Activins, members of transforming growth factor β (TGF-β) superfamily, were first isolated from porcine ovarian follicular fluid and identified as activating factors for the release of follicle stimulating hormone. Activins function both in autocrine and paracrine manner. They conduce signalling by binding to extracellular domains of type I and type II receptors and allowing the kinase domains of type II receptors to phosphorylate those of type I receptors and initiate the intracellular signalling. Activins, like all other members in the TGF-β superfamily, are synthesized as larger precursors. During the secretory pathway, the precursors are processed by furin-like proteases that cleave the polypeptide after a dibasic recognition sequence between the pro- and mature domains, releasing the mature signalling domain from the covalent linkage to the pro-domain12.

As we had engineered an HRV 3C protease cleavage site into our protein, we could mimic the furin processing of pro-activin A in vitro. SEC-MALS analysis shows that after the cleavage the pro- and mature domains remain associated with each other, eluting at the same volume as the uncleaved protein and showing dimeric molecular weight of 88.3 kDa. In contrast to the uncleaved precursor, the cleaved pro-activin A complex is highly active in the cell-based luciferase assay with a half-maximal response concentration (EC50) of 29±3 pM (all the EC50 and IC50 values and their s.d. values are determined from three replicates). The complex-derived mature activin A conducts signalling marginally better than the pro-mature complex, with an EC50 value of 20±2 pM, which is in excellent agreement with the activity of our control activin A (EC50=21±2 pM). These data confirm that the refolded and proteolytically cleaved pro-activin A is correctly folded, homogenous and fully biologically active and that the pro-domain has only a marginal effect on the bioactivity. The structure of the cleaved pro-activin A complex was determined at 2.85 Å by molecular replacement using the precursor structure as our starting model. The linker between the pro- and mature domains, with the protease cleavage site, is visible neither in the precursor nor in the pro-mature complex. The palm α-helix of the mature domain appears to be disordered in both pro-domain structures, lacking interpretable electron density. With low nanomolar affinity, and considering the EC50 of 20–30 pM, it is likely that the pro-activin A complex has mostly dissociated at the concentrations required for full bioactivity. The response curves of FST-288 binding to the mature activin A and cleaved pro-activin A complex reached the equilibrium very quickly at 25 nM analyte concentration, resulting in very similar Kd values of 209.0±0.6 and 258.6±1.2 pM, respectively.

>MSHHHHHHSMSAAPDSPSSALAALPKDVPNSQPEMVEAVKKHILNMLHLKKRPDVTQPVPKAALLNAIRKLHVGKVGENGYVEIEDDIGRRAEMNELMEQTSEIITFAESGTARKTLHFEISKEGSDLSVVERAEVWLFLKVPKANRTRTKVTIRLFQQQKHPQGSLDTGEEAEEVGLKGERSELLLSEKVVDARKSTWHVFPVSSSIQRLLDQGKSSLDVRIACEQCQESGASLVLLGEEKEQSHRPFLMLQARQSEDHPHLEVLFQGP[4x];>[4x]GLECDGKVNICCKKQFFVSFKDIGWNDWIIAPSGYHANYCEGECPSHIAGTSGSSLSFHSTVINHYRMRGHSPFANLKSCCVPTKLRPMSMLYYDDGQNIIKKDIQNMIVEECGCS> MP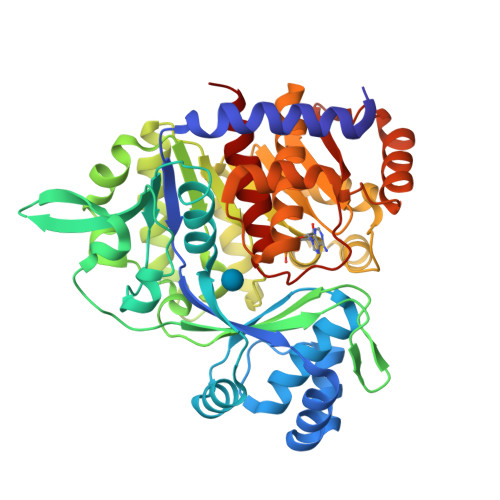TWEELYKNAIEKAIKSVPKVKGVLLGYNTNIDAIKYLDSKDLEERIIKAGKEEVIKYSEELPDKINTVSQLLGSILWSIRRGKAAELFVESCPVRFYMKRWGWNELRMGGQAGIMANLLGGVYGVPVIVHVPQLSRLQANLFLDGPIYVPTLENGEVKLIHPKEFSGDEENCIHYIYEFPRGFRVFEFEAPRENRFIGSADDYNTTLFIREEFRESFSEVIKNVQLAILSGLQALTKENYKEPFEIVKSNLEVLNEREIPVHLEFAFTPDEKVREEILNVLGMFYSVGLNEVELASIMEILGEKKLAKELLAHDPVDPIAVTEAMLKLAKKTGVKRIHFHTYGYYLALTEYKGEHVRDALLFAALAAAAKAMKGNITSLEEIREATSVPVNEKATQVEEKLRAEYGIKEGIGEVEGYQIAFIPTKIVAKPKSTVGIGDTISSSAFIGEFSFTL N,N'-ethane-1,2-diylbis(2-iodoacetamide) | C6 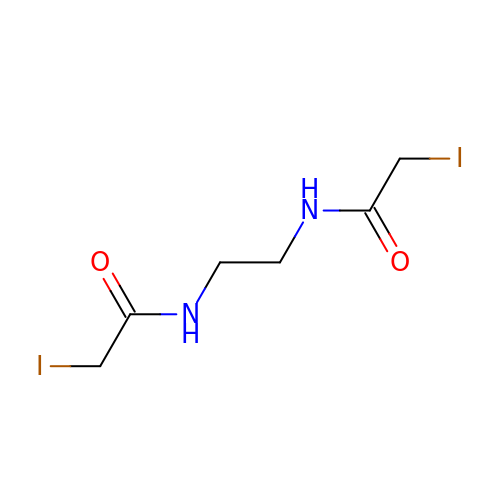H10 I2 N2 O2 | RLFPCLMBTQOMLI-UHFFFAOYSA-N3-(2-{[(4-chlorophenyl)carbamoyl]amino}propan-2-yl)-N-hydroxybenzene-1-carboximidamide 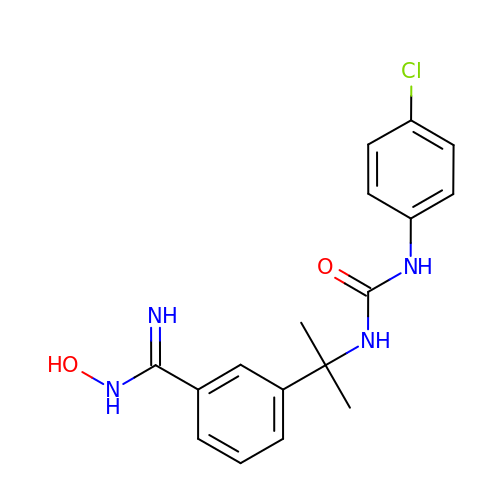| C17 H19 Cl N4 O2 | NZOIAPIDYRJDOM-UHFFFAOYSA-N> SMIKQRTLKNIIRATGVGLHSGEKVYLTLKPAPVDTGIVFCRTDLDPVVEIPARAENVGETTMSTTLVKGDVKVDTVEHLLSAMAGLGIDNAYVELSASEVPIMDGSAGPFVFLIQSAGLQEQEAAKKFIRIKREVSVEEGDKRAVFVPFDGFKVSFEIDFDHPVFRGRTQQASVDFSSTSFVKEVSRARTFGFMRDIEYLRSQNLALGGSVENAIVVDENRVLNEDGLRYEDEFVKHKILDAIGDLYLLGNSLIGEFRGFKSGHALNNQLLRTLIADK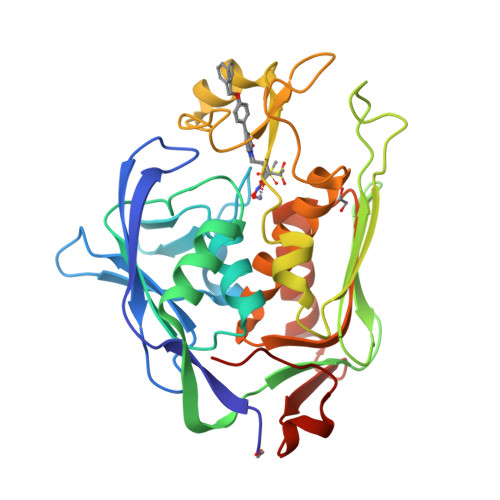DAWEVVTFEDARTAPISYMRPAAAV> MVSNTTPIVELKGDANTLKCLRYRFKKHSTLYTAVSSTWHWTGHNVKHKSAIVTLTYDS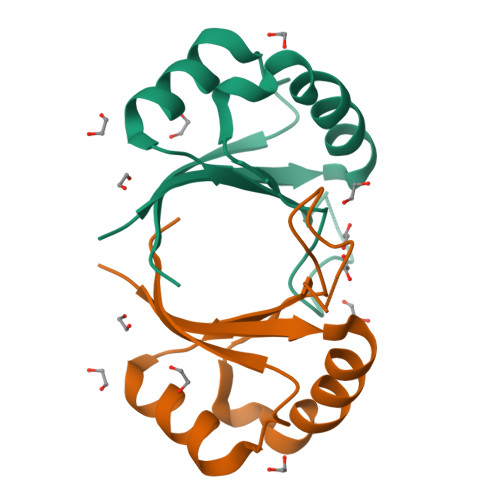EWQRDQFLSQVKIPKTITVSTGFMSI> PELPEVETVRRELEKRIVGQKIISIEATYPRMVLTGFEQLKKELTGKTIQGISRRGKYLIFEIGDDFRLISHLRMEGKYRLATLDAPREKHDHLTMKFADGQLIYADVRKFGTWELISTDQVLPYFLKKKIGPEPTYEDFDEKLFREKLRKSTKKIKPYLLEQTLVAGLGNIYVDEVLWLAKIHPEKETNQLIESSIHLLHDSIIEILQKAIKLGGSSIRTYSALGSTGKMQNELQVYGKTGEKCSRGHGAEIQKIKVAGRGTHFCPVCQQK

The Fpg/Nei superfamily (also called H2TH superfamily) includes bi-functional enzymes able to remove a wide variety of oxidized bases. The enzyme architecture consists in two globular domains connected by a flexible hinge: (i) a N-terminal domain rich in β-structures containing a highly conserved N-terminal α-helix (αA) displaying generally a proline (P1) at the N-terminal involved in catalysis and (ii) a C-terminal domain rich in α-structures containing both DNA binding domains of the enzyme (the H2TH motif and a β-hairpin domain structured in most cases as a Zinc finger). All these enzymes feature AP lyase activity consisting in the successive cleavage at the 3’ and then at the 5’ sides of the abasic (AP) site according to β,δ-elimination. In this work, we deciphered at the atomic level the structural and/or functional determinants required for the specific inhibition of ZnF Fpg/Nei DNA glycosylases by the uncompetitive inhibitor 2TX.

Four LlFpg variants were constructed: W179A, R247G, C248GH and C268H. The aim of constructing these point mutations was to (i) disrupt the 2TX binding site (W179A), (ii) increase the C268 thiolate reactivity (R247G) or (iii)inactivate the reactive sites C248 or C268 by replacing C to H (C248GH, which mimics the situation found in hNEIL2, Supplementary Figure S1c; C268H). The crystal structures of R247G and C248GH bound to 14-mer THF-DNA have been solved and indicate that these point mutations do not affect the overall structure of ZnF as compared to the wild-type enzyme. To evaluate the 2TX sensitivity of R247G and C248GH, we used the PAR assay. In contrast, the variant C248GH appears about two times less sensitive to 2TX than the wild type. As seen in the crystal structure of [WT/THF]-2TX, this suggests that C248 is one of the reactive targets of 2TX but not the only one since C248GH remains sensitive to 2TX. This result is in perfect agreement with the crystal structure of [WT/Bz]-2TX showing that C268 is another reactive target for 2TX and with the observation that hNEIL2 containing CHC2 type of ZnF is also inhibited by 2TX.>[2x]GAMSTTSTTIQVIGAGLPRTGTNSMKKALEIIYSKPCYHMYEIIFKKQSDISIWQQLIDETHKTTSDKRKIYNGLNELLNGYIATTDLPSCSFYKELMTMYPNAKVLLTIRDKYDWLYSLRKVVLPKSTDPWKLKIEEGDQVLGIDSNFYKMSEDSLKFAFQKNH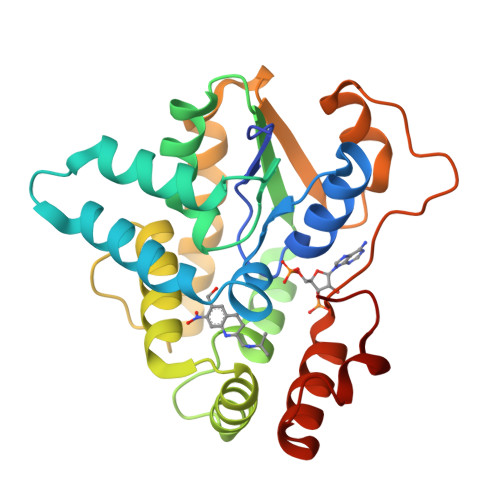INLDDDEILLECYDEYNRLVQEIVPPERLLIHHLGDGWESLCQFLNVDIPNGISYPCANSHHQMTQLTEQLIKHKSLDDIIHMFPGLI> VQVLITDSGQRTGTGSALMAMKDAGVNTYRWQGGEQRPATIISEPDRNVRYARLAGDFAASVKAGEESVAQVSGVREQAILTQAIRSELKTQGVLGHPEVTMTALSPVWLDSRSRYLRDMYRPGMVMEQWNPETRSHD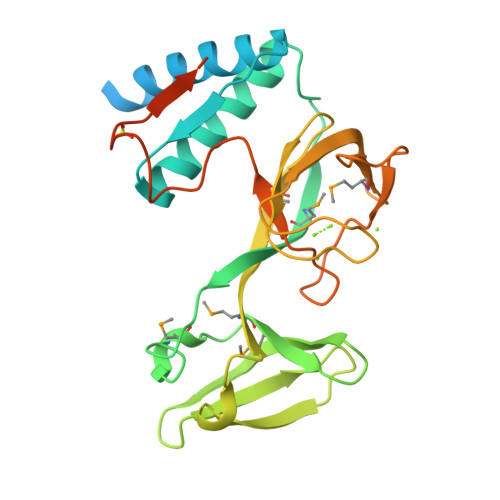RYVIDRVTAQSHSLTLRDAQGETQVVRISSLDSSWSLFRPEKMPVADGERLRVTGKIPGLRVSGGDRLQVASVSEDAMTVVVPGRAEPASLPVSDSPFTALKLENGWVETPGHSVSDSATVFASVTQMAMDNATLNGLARSGRDVRLYS>[2x]RAP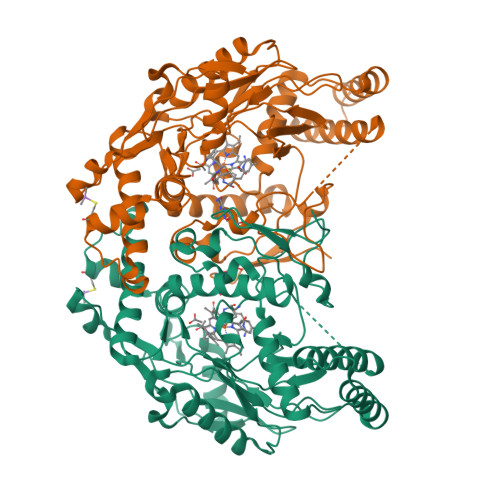APATPHAPDHSPAPNSPTLTRPPEGPKFPRVKNWELGSITYDTLCAQSQQDGPCTPRRCLGSLVLPRKAQTRPSPGPPPAEQLLSQARDFINQYYSSIKRSGSQAHEERLQEVEAEVASTGTYHLRESELVFGAKQAWRNAPRCVGRIQWGKLQVFDARDCSSAQEMFTYICNHIKYATNRGNLRSAITVFPQRAPGRGDFRIWNSQLVRYAGYRQQDGSVRGDPANVEITELCIQHGWTPGNGRFDVLPLLLQAPDEAPELFVLPPELVLEVPLEHPTLEWFAALGLRWYALPAVSNMLLEIGGLEFSAAPFSGWYMSTEIGTRNLCDPHRYNILEDVAVCMDLDTRTTSSLWKDKAAVEINLAVLHSFQLAKVTIVDHHAATVSFMKHLDNEQKARGGCPADWAWIVPPISGSLTPVFHQEMVNYILSPAFRYQPDPW4-[(6-CHLORO-1-BENZOTHIEN-2-YL)SULFONYL]-1-{[1-(2-HYDROXYETHYL)-1H-PYRROLO[3,2-C]PYRIDIN-2-YL]METHYL}PIPERAZIN-2-ONE 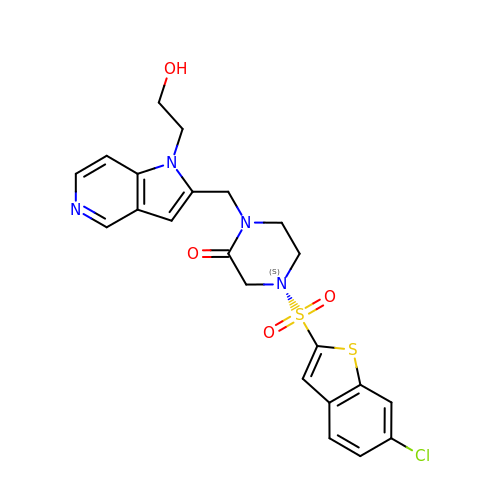| C22 H21 Cl N4 O4 S2 | NZNFLUOJACWZKX-UHFFFAOYSA-N>[12x]MPKSFYDAVGGAKTFDAIVSRFYAQVAEDEVLRRVYPEDDLAGAEERLRMFLEQYWGGPRTYSEQRGHPRLRMRHAPFRISLIERDAFLRCM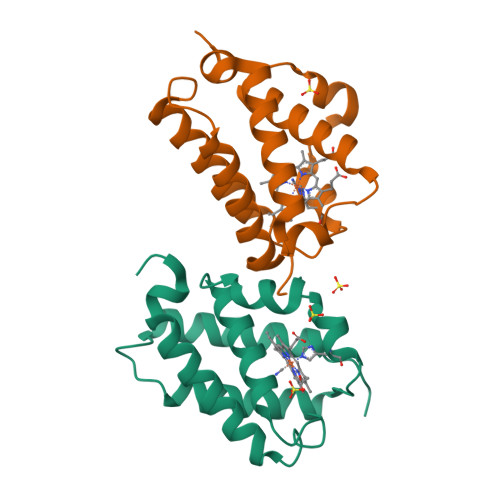HTAVASIDSETLDDEHRRELLDYLEMAAHSLVNSPF>MKVVDISKINELVKEGATLMIGGFLGVGTPENIIDEIIRHNISNLTVIANDTAFEDRGIGKLVKNKLCKKVIVSHIGTNPETQRQMIEGTLEVELVPQGTLAERIRAAGVGLGGILTPTGVGTVVEKDKKVIEVEGKKYLLELPIHADVALIKAKKADYLGNLVYNLTAENFNPIMALAAKTVIAEVEEIVPTGTLSPNEIKTPGIIVDYIVTGVTR[2x];>MNPKEKIAIRVAQELKKGQLVNLGIGLPTLVANYIPKDIHVFFQSENGIIGMGPAPKEGYENSDLTNAGASYITALPGAMTFDSAFSFGIIRGGHLDVTVLGGLQVDEEGHLANWMIPGKMIPGMGGAMDLVTGAKKVIVAMTHTAKGTPKIVKKCTLPLTSIRKVDLIVTELAVIEPTDEGLLLKEISKETTLDEVLKLTEAKLIIADDLKIFA[2x]

CtfAB then transfers the CoA from acetoacetyl-CoA to acetate to reform an acetyl-CoA and produce acetoacetate. CtfAB is a member of family 1 CoA transferases. CtfB contains the acetyl-CoA binding site and the PS01724 signature sequence which includes the catalytic glutamate residue (E46) sandwiched between two short antiparallel beta strands on the N-terminal end of an eight-stranded mixed beta sheet. CtfA contains the acetate binding site and the PS01723 signature sequence.

Acetate molecules were identified in every CtfAB structure in the substrate-binding pocket directly adjacent to catalytic residue E46. Acetate 1, colored magenta, is the only location where acetate is bound in the same conformation in each structure. The conserved acetate-binding site in Wt-CtfAB is shown in Figure 4. L25 and F24 of CtfA form a hydrophobic pocket for the methyl group of acetate (301 A). The methyl group of acetate (301 A) is 3.9 Å from the CZ side chain carbon of F24 and 4.0 Å from the CD2 atom of L25. On the opposite side of the binding site, one of the polar oxygens is in good hydrogen bonding distance (2.5 Å) to the side chain NE of CtfA Q98 and 3.4 Å to the side chain ND2 of CtfA N50. The second polar oxygen of acetate is 3.0 Å from the OE2 side chain atom of the catalytic E46 residue. This oxygen is solvent exposed and connected to an extensive water-filled cavity. In T. mel CtfA, there is a contiguous hydrophobic patch between F24, L25, the methyl group of T78, and F54. This hydrophobic patch could provide both binding affinity for acetate and improved thermal stability. While it is clear from SEC and native-PAGE that multiple higher order oligomeric states of CtfAB do exist in solution, the heterotetramer is the highest-ordered state apparent in CtfAB crystals.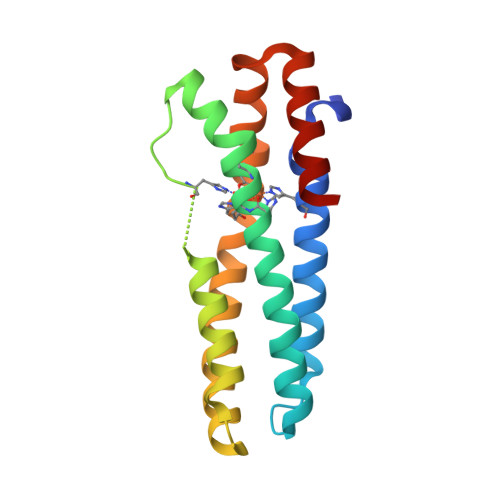>[4x]MAPFPEEVDVFTAPHWRMKQLVGLYCDKLSKTNFSNNNDFRALLQSLYATFKEFKMHEQIENEYIIGLLQQRSQTIYNVHSDNKLSEMLSLFEKGLKNVKNEYEQLNYAKQLKERLEAFTRDFLPHMKEEEEVFQPMLMEYFTYEELKDIKKKVIAQHCSQ> SRLDKSKVINSALELLNEVGIEGLTTRKLAQKLGVEQPTLYWHVKNKRALLDALAIEMLDRHHTHFCPLEGESWQD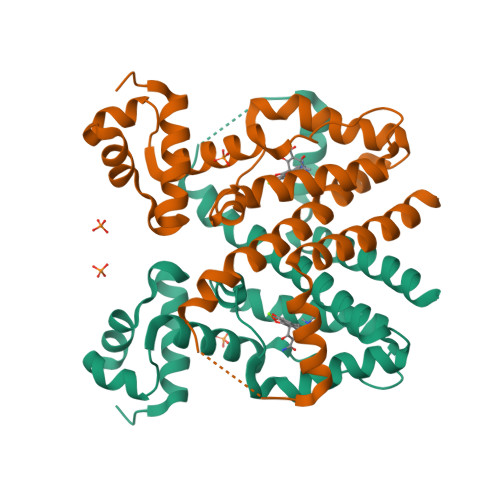FLRNNAKSFRCALLSHRDGAKVHLGTRPTEKQYETLENQLAFLCQQGFSLENALYALSAVGHFTLGCVLEDQEHQVAKEERETPTTDSMPPLLRQAIELFDHQGAEPAFLFGLELIICGLEKQLKC N-{3-CYANO-6-[3-(1-PIPERIDINYL)PROPANOYL]-4,5,6,7-TETRAHYDROTHIENO[2,3-C]PYRIDIN-2-YL}1-NAPHTHALENECARBOXAMIDE 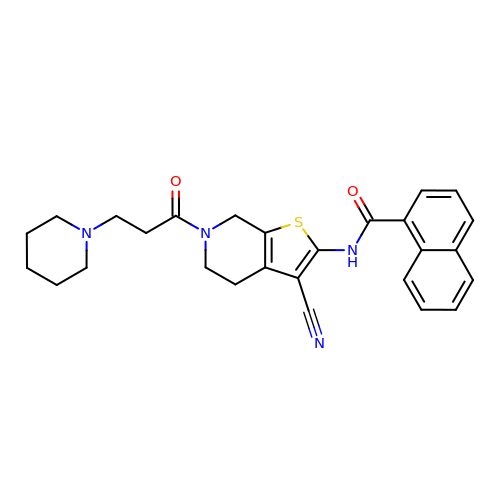| C27 H28 N4 O2 S | PRZGSWGFNRYBIP-UHFFFAOYSA-N>AHHHHHHSAAENLYFQGEFNILLATDSYKVTHYKQYPPNTSKVYSYFECREKKTENSKLRKVKYEETVFYGLQYILNKYLKGKVVTKEKIQEAKDVYKEHFQDDVFNEKGWNYILEKYDGHLPIEIKAVPEGFVIPRGNVLFTVENTDPECYWLTNWIETILVQSWYPITVATNSREQKKILAKYLLETSGNLDGLEYKLHDFGYRGVSSQETAGIGASAHLVNFKGTDTVAGLALIKKYYGTKDPVPGYSVPAAEHSTITAWGKDHEKDAFEHIVTQFSSVPVSVVSDSYDIYNACEKIWGEDLRHLIVSRSTQAPLIIRPDSGNPLDTVLKVLEILGKKFPVTENSKGYKLLPPYLRVIQGDGVDINTLQEIVEGMKQKM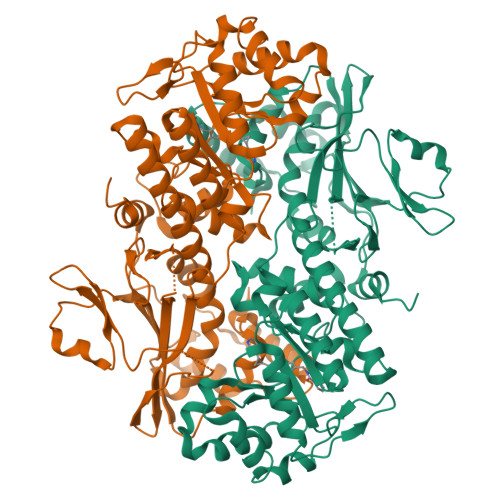WSIENIAFGSGGGLLQKLTRDLLNCSFKCSYVVTNGLGINVFKDPVADPNKRSKKGRLSLHRTPAGNFVTLEEGKGDLEEYGQDLLHTVFKNGKVTKSYSFDEIRKNAQLNIE[2x]> MAGAQDFVPHTADLAELAAAAGECRGCGLYRD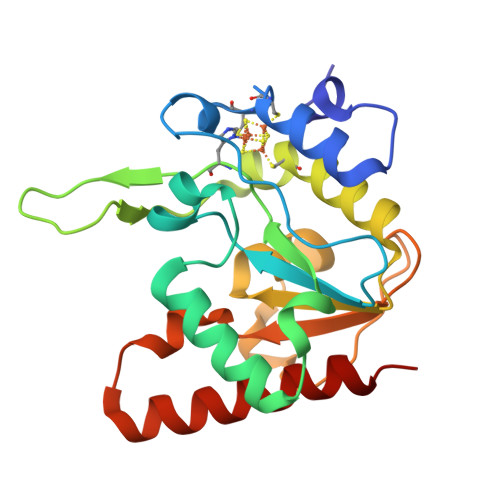ATQAVFGAGGRSARIMMIGQQPGDKEDLAGLPFVGPAGRLLDRALEAADIDRDALYVTNAVKHFKFTRAAGGKRRIHKTPSRTEVVACRPWLIAEMTSVEPDVVVLLGATAAKALLGNDFRVTQHRGEVLHVDDVPGDPALVATVHPSSLLRGPKEERESAFAGLVDDLRVAADVRP> MRGVVGVLALQGDFREHKEALKRLGIEAKEVRKKEHLEGLKALIVPGGESTTIGKLAREYGIEDEVRKRVEEGSLALFGTCAGAIWLAKEIVGYPEQPRLGVLEAWVERNAFGRQVESFEEDLEVEGLGSFHGVFIRAPVFRRLGEGVEVL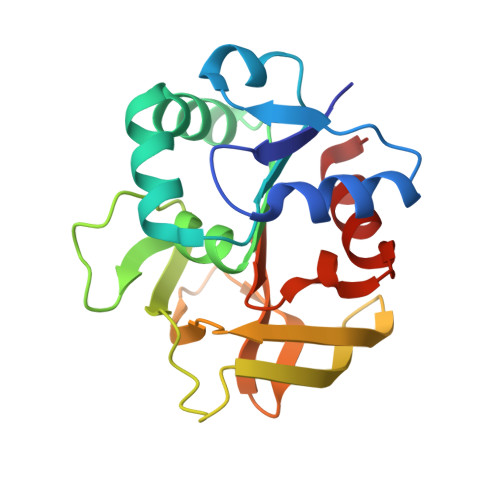ARLGDLPVLVRQGKVLASSFHPELTEDPRLHRYFLELAGV>SKKIGLFYGTQTGKTKSVAEIIRDEFGNDVVTLHDVSQAEV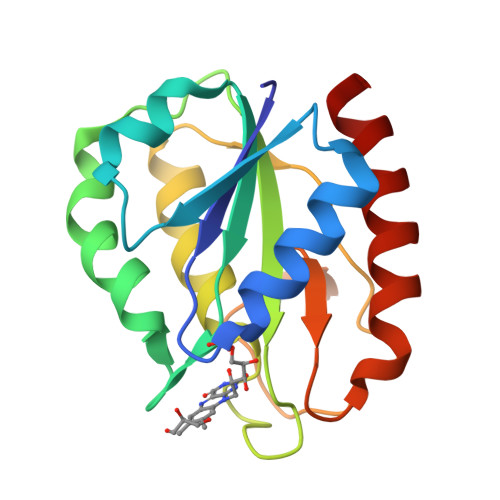TDLNDYQYLIIGCPTWNIGKLQSDWEGLYSELDDVDFNGKLVAYFGTGDQIGYADNFQDAIGILEEKISQRGGKTVGYWSTDGYDFNDSKALRNGKFVGLALDEDNQSDLTDDRIKSWVAQLKSEFGL[4x]> MENLNHSPLEDIKVNPWKTPQSTARVITLRVEDPNEINNLLSINEIDNPNYILQAIMLANAFQNALVPTSTDFGDALRFSMPK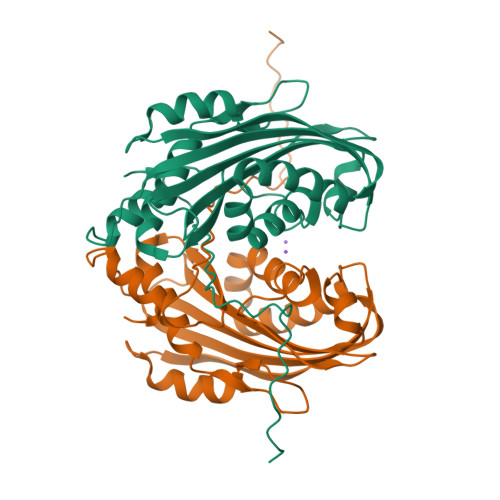GLEIANTITPMGAVVSYVDQNVTQTNNQVSVMINKVLEVLKTVLGVALSGSVIDQLTAAVTNTFTNLNTQKNEAWIFWGKETANQTNYTYNVLFAIQNAQTGGVMYCVPVGFEIKVSAVKEQVLFFTIQDSASYNVNIQSLKFAQPLVSSSQYPIADLTSAINGTL>MSLKIIAPTDKTITPSGTWSIGARAGDFVFIGGMHGTDRVTGKMVDGDEARIRRMFDNMLAAAEAAGATKADAVRLTVFVTDVAKYRPVVNKVQKDIWGDGPYPPRTVLQVPALDQGDIAEIDGTFYAPAEGH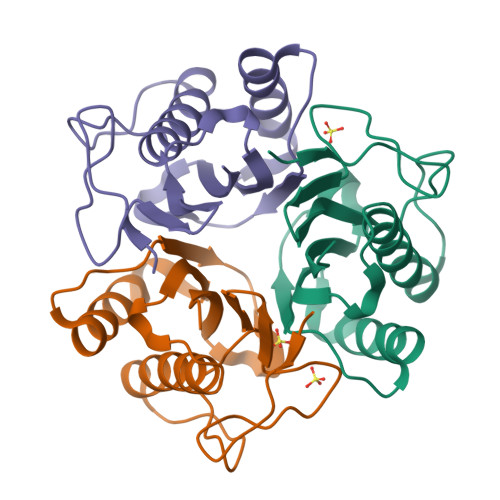HHHHH[12x]> MWRRHYKLVPQIDTR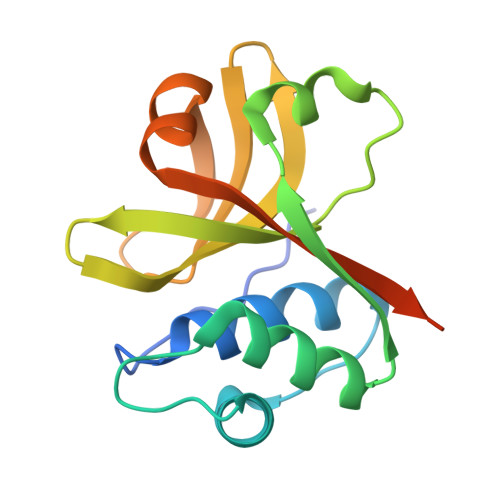DCGPAVLASVAKHYGSNYSIAYLRELSKTNKQGTTALGIVEAAKKLGFETRSIKADMTLFDYNDLTYPFIVHVIKGKRLQHYYVVYGSQNNQLIIGDPDPSVKVTRMSKERFQSEWTGLAIFLAPQPNYKPHKGEHHHHHH4-({(1S)-2-(azetidin-1-yl)-1-[4-chloro-3-(trifluoromethyl)phenyl]ethyl}amino)quinazoline-8-carboxamide | C21 H19 Cl F3 N5 O | 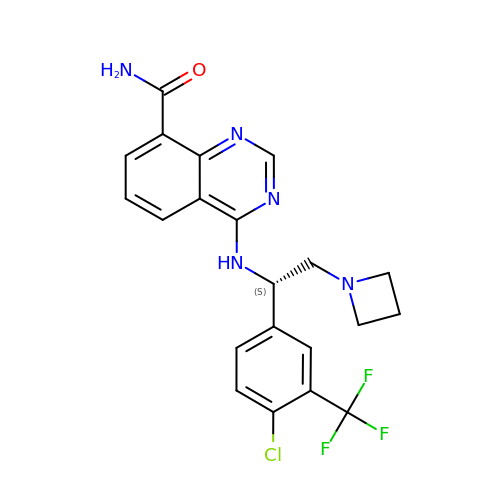HXAUJHZZPCBFPN-QGZVFWFLSA-N>LRVGFIGFGEVAQTLASRLRSRGVEVVTSLEGRSPSTIERARTVGVTETSEEDVYSCPVVISAVTPGVALGAARRAGRHVRGIYVDINNISPETVRMASSLIEKGGFVDAAIMGSVRRKGADIRIIASGRDAEEFMKLNRYGLNIEVRGREPGDASAIKMLRSSYTKGVSALLWETLTAAHRLGLEEDVLEMLEY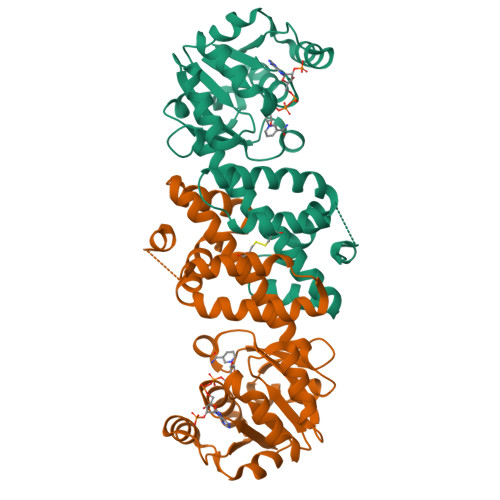TEGNDFRESAISRLKSSCIHARRRYEEMKEVQDMLAEVIDPVMPTCIIRIFDKLKDVKVSADARLQGCA[2x]> MKDLVDTTEMYLRTIYELEEEGVTPLRARIAERLEQSGPTVSQTVARMERDGLVVVASDRSLQMTPTGRTLATAVMRKHRLAERLLTDIIGLDINKVHDEASRWEHVMSDEVERRLVKVLKDVSRSPFGNPIPGLDELGVGNSDAAAPGTRVIDAATSMPRK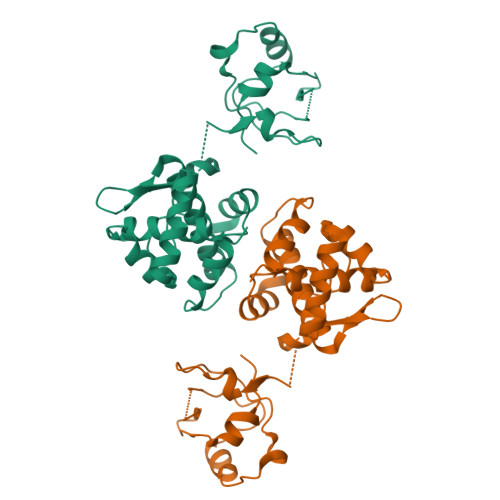VRIVQINEIFQVETDQFTQLLDADIRVGSEVEIVDRDGHITLSHNGKDVELLDDLAHTIRIEEL> GAMGQTSQQDEST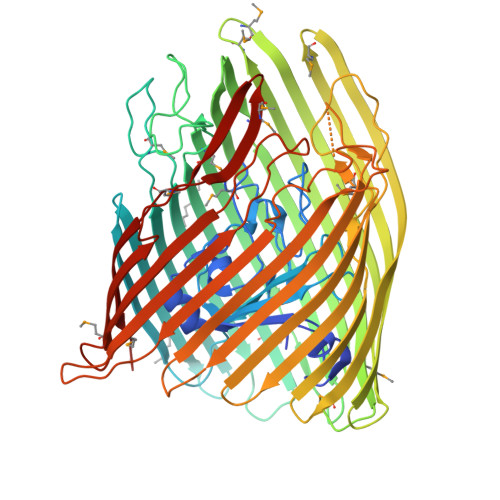LVVTASKQSSRSASANNVSSTVVSAPELSDAGVTASDKLPRVLPGLNIENSGNMLFSTISLRGVSSAQDFYNPAVTLYVDGVPQLSTNTIQALTDVQSVELLRGPQGTLYGKSAQGGIINIVTQQPDSTPRGYIEGGVSSRDSYRSKFNLSGPIQDGLLYGSVTLLRQVDDGDMINPATGSDDLGGTRASIGNVKLRLAPDDQPWEMGFAASRECTRATQDAYVGWNDIKGRKLSISDGSPDPYMRRCTDSQTLSGKYTTDDWVFNLISAWQQQHYSRTFPSGSLIVNMPQRWNQDVQELRAATLGDARTVDMVFGLYRQNTREKLNSAYDMPTMPYLSSTGYTTAETLAAYSDLTWHLTDRFDIGGGVRFSHDKSSTQYHGSMLGNPFGDQGKSNDDQVLGQLSAGYMLTDDWRVYTRVAQGYKPSGYNIVPTAGLDAKPFVAEKSINYELGTRYETADVTLQAATFYTHTKDMQLYSGPVRMQTLSNAGKADATGVELEAKWRFAPGWSWDINGNVIRSEFTNDSELYHGNRVPFVPRYGAGSSVNGVIDTRYGALMPRLAVNLVGPHYFDGDNQLRQGTYATLDSSLGWQATERMNISVYVDNLFDRRYRTYGYMNGSSAVAQVNMGRTVGINTRIDFF> MASDGYTIKPNKKVTYSALGEDERMIGFSYKDFGISSSEKITEVQVNISANKNIGKYVGQFGTSTTDSANGYWAMGDEITQSISGNSGTITWKVPSDISSIIQTQYG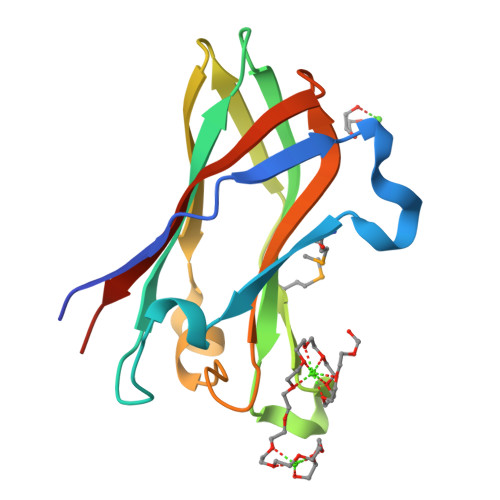GEIKFGVWWIDCDEFTIDSVVLKLEHHHHHH> KIWQSRRKTLEEEKASDWQIELNGTLFDSELQPGSSFKAEGFRKVTDKLKINYLPHRRRVHQPLNTVNIHNERNEYTPELCQREESSNKEPSDSVPQEVSSSRDNRASNRRFQQDIEAQKAAIGTESELLSLNQLNK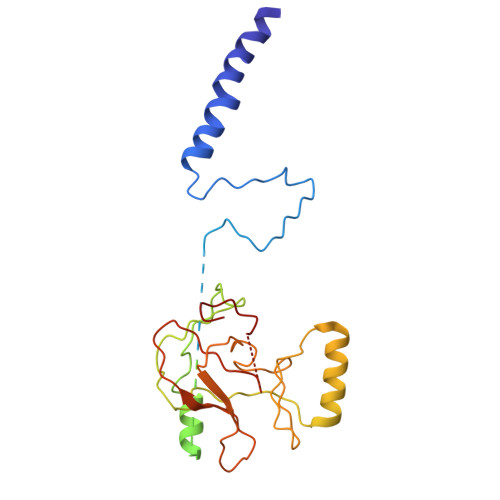RKKPVMFARSAIHNWGLYALDSIAAKEMIIEYVGERIRQPVAEMREKRYLKNGIGSSYLFRVDENTVIDATKKGGIARFINHCCDPNCTAKIIKVGGRRRIVIYALRDIAASEELTYDYKFEREKDDEERLPCLCGAPNCK> RQLALEAKGETPSAVTRLSVVAKSEPQDEQSRSQSPRRIILSRLKAGEVDLLEEELGHLTTLTDVVKGADSLSAILPGDIAEDDITAVLC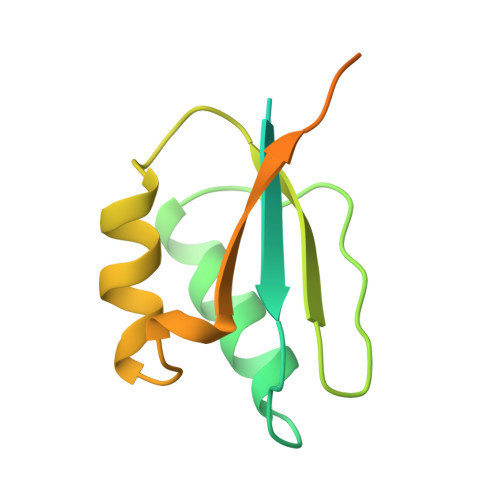FVIEADQITFETVEVSPKISTPPVLKLAAEQAPTGRVEREKTTR> GSHMASPNGQTKPLPALKLALEYIVPCMNKHGICVVDDFLGKETGQQIGDEVRALHDTGKFTDGQLVSQKSDSSKDIRGDKITWIEGKEPGCETIGLLMSSMDDLIRHCNGKLGSYKIKERTKAMVACYPGNGTGYVRHVDNPNGDGRCVTCIYYLNKDWDAKVSGGILRIFPEGKAQFADIEPKFDRLLFFWSDRRNPHEVQPAYATRYAITVWYFDADERARAKVKYLTGEKGVRVELNKPSDSVGKDVF

The ferrous iron and 2-oxoglutarate (2OG)-dependent HIF prolyl hydroxylases (PHDs/EGLNs) catalyse trans-4-prolyl hydroxylations on HIFα subunits, thus promoting their binding to the von Hippel–Lindau protein (VHL), a targeting component of a ubiquitin E3 ligase, and signalling for HIFα degradation under normoxic conditions. The PHD-catalysed hydroxylations of HIF-1α/HIF-2α in higher animals occur in amino- and carboxy-terminal oxygen-dependent degradation domains (NODD and CODD). The three human PHDs exhibit different NODD/CODD selectivities, with PHD3 being substantially more selective for CODD than PHD1/2 (refs 16). Biophysical analyses employing crystallography and NMR reveal that the molecular basis of PHD isoform and variant selectivity involves enzyme–substrate interactions involving β2/β3 loop residues (that bind the LXXLAP motif) and helices α3 and α4, regions which display sequence variations between the PHD isoforms.

Using biochemical and structural studies, we identified four more residues in α3 and α3-βI loop regions (PHD2/Ile280, Arg281, Ile292 and Gly294 that are substituted in PHD3/Val102, Leu103, Val114 and Glu116, respectively) and which play roles in determining selectivity. Indeed, we found that FG2216 (IOX3)35, used in clinical trials for treatment of anaemia, preferentially displaces NODD over CODD from PHD2.> ISGGDAIYSSTGRCSLGFNVRSGSTYYFLTAGHCTDGATTWWANSARTTVLGTTSGSSFPNNDYGIVRYTNTTIPKDGTVGGQDITSA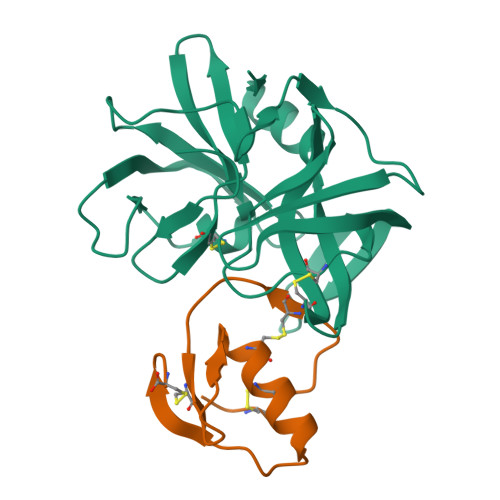ANATVGMAVTRRGSTTGTHSGSVTALNATVNYGGGDVVYGMIRTNVCAEPGDSGGPLYSGTRAIGLTSGGSGNCSSGGTTFFQPVTEALVAYGVSVY;> VDCSEYPKPACTVEYRPLCGSDNKTYGNKCNFCNAVVESNGTLTLSHFGKC> 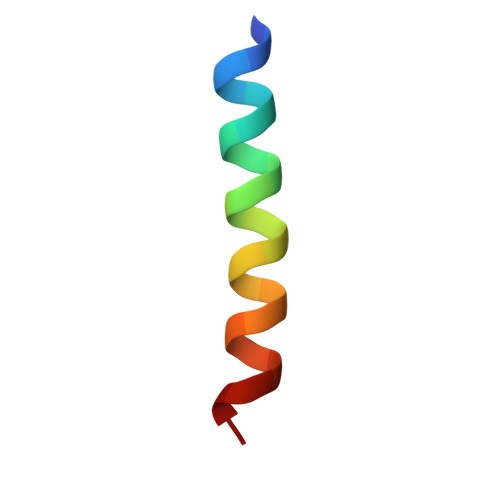RPEIWAAQEIRRIGDENNAYYAR1-[3-[(4-chloranyl-2-fluoranyl-phenyl)carbamoylamino]-4-[cyclohexyl(2-methylpropyl)amino]phenyl]pyrrole-2-carboxylic acid | C28 H32 Cl F N4 O3 | 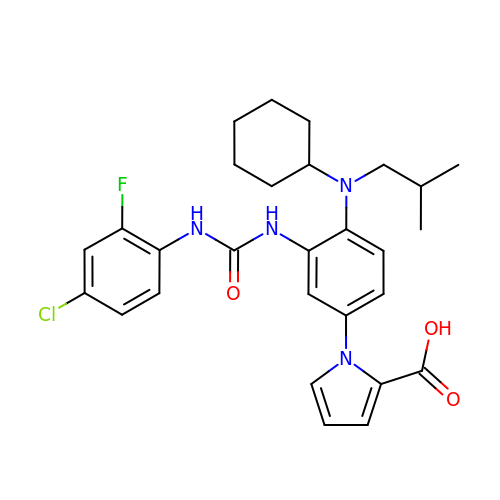JYDXSLBOQXZAKM-UHFFFAOYSA-N>[4x]HHHHHHENLYFQGPNPAGQLTFTQLCMSGDGYYQHRTNLIYSGGFVQHYSGSWAVTEYGSKFKKVDEYATALWRNVYANELKNVVDIIKNTSNDPAASNMNAVAKIMKVMVAQRLTDIYGDVPYSEAGLGFSQGIVTPKYDKQQDIYNSFFKDLDESFTQLNASGGSVKGDLFYNGDISKWKKLANTMRLRLAMRISEVSPAEAEKQAKAAFQNGVFESNDDNCLMHHLDFPFNDNPATLDFRGNGLSYGFISDEHGDHFSSLLIDYLRDNGDPRLKMLATPKTGSVNGGPIGPGEELYEGVRPGVFRWEVVGGSNAASGIQPYLKLRTTPFLHVSYSESQLLLAEAAYRGWVAGSAADFYKKGVEAGIKQLEVYGAAPASQASIDAYVNAKPLAAGTEKEQIGTQLWITYLFNSIEAYSNWRRTGYPHLLPITNSDSQTGGVVPTRLYYPNDEMQKNEKNYMEAVQRMGGTNDWTGKVWWDVN

The studied chitin utilization locus (ChiUL) is encoded by the soil saprophyte Flavobacterium johnsoniae, which is a Bacteroidetes member exhibiting gliding motility. The ChiUL of F. johnsoniae consists of eleven genes that encode four enzymes, a predicted inner membrane transporter, a predicted two-component sensor/regulator system (TCS), and two individual SusC/D-like pairs (CusC/D, chitin utilization system). The SusC/D-like pairs are believed to be specific for their cognate carbohydrate targets, and act in concert to bind (SusD) and transport (SusC) oligosaccharides across the outer membrane. The resulting ChiOs, and likely chitin crystals as well (analogous to the archetypal starch-binding SusD protein of B. thetaiotaomicron), are captured by the CusD proteins.

CusDI and CusDII exhibit comparatively low sequence identity (27%) and may thus have different carbohydrate affinity characteristics. In contrast, CusDII only bound chitopentaose and chitohexaose, with 10-fold higher affinity for the latter. It is likely that both CusD proteins are able to bind even longer chitin fragments, which due to solubility issues are not amenable to ITC analysis. Despite considerable efforts, crystals with bound ChiO ligands were not obtained, likely due to crystal packing, which for both proteins affected the predicted ligand-binding site. The overall structures of CusDI and CusDII overlay with an RMSD of 2.2 Å for 363 Cα pairs and display the canonical SusD protein fold featuring four tetratricopeptide repeats that act as a structural scaffold. The most striking feature of the putative substrate-binding regions of both CusDI and CusDII is the presence of two Trp residues that would provide a flat platform for binding ChiOs as well as insoluble chitin, as has been observed in chitin-binding carbohydrate-binding modules (CBMs). CusDI features W280 and W65, whereas CusDII displays W330 and W74 that are located at non-equivalent positions but may nevertheless have similar roles. While both glycan-binding platforms overlay within the known glycan-binding site of SGBP-A, they are offset from each other, suggesting that ChiOs are bound differently by each protein. The area of CusDI surrounding W280 and W65 displays several residues that may provide hydrogen-bonding or electrostatic interactions with individual GlcNAc residues of chitin, while there are fewer such residues within the aromatic interface of CusDII. This may account for the difference in binding specificity and affinity between the two proteins.> RSWHYVEPKFLNKAFEVALKVQIIAGFDRGLVKWLRVHGRTLSTVQKKALYFVNRRYMQTHWA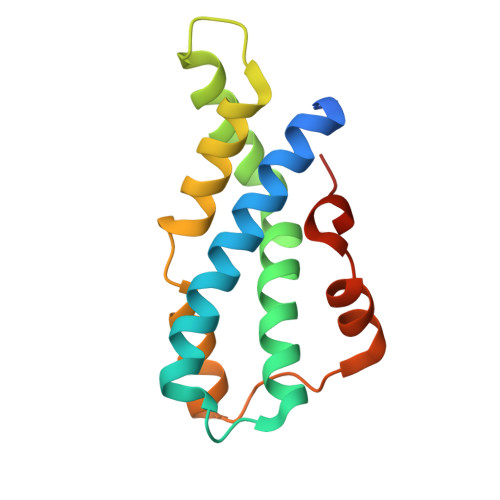NYMLWINKKIDALGRTPVVGDYTRLGAEIGRRIDMAYFYDFLKDKNMIPKYLPYMEEINRMRPADVPVKYMGK> MAAHQLSDFQRNKILRVFNTFYDCNHD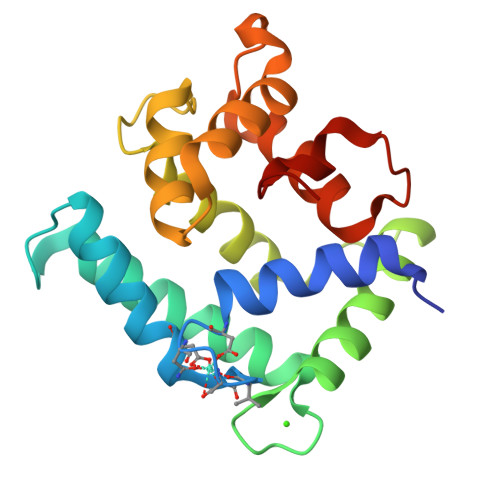GVIEWDDFELAIKKICNLHSWPTDGKKHNEARATLKLIWDGLRKYADENEDEQVTKEEWLKMWAECVKSVEKGESLPEWLTKYMNFMFDVNDTSGDNIIDKHEYSTVYMSYGIPKSDCDAAFDTLSDGGKTMVTREIFARLWTEYFVSNDRGAKGNHLFGTLKL>TDSLLSLVLPDRVASAEVYDDPPGLSPLPEEEPLIARSVAKRRNEFVTVRYCARQALGELGVGPVPILKGDKGEPCWPDGVVGSLTHCQGFRGAVVGRSTDVRSVGIDAEPHDVLPNGVLDAITLPIERAELRGLPGDLHWDRILFCAKE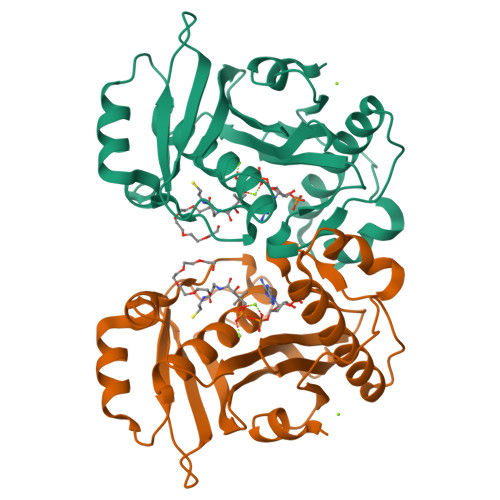ATYKAWYPLTHRWLGFEDAHITFEVDGSGTAGSFRSRILIDPVAEHGPPLTALDGRWSVRDGLAVTAIVLLEH[2x]2-hydroxy-N-[(1S)-1-hydroxy-3-oxopropyl]-L-aspartic acid | C7 H11 N O7 | 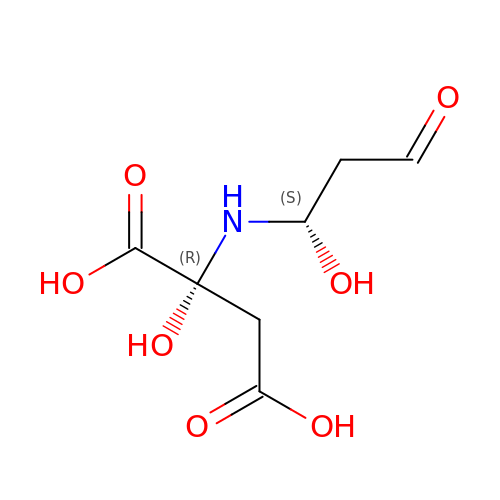CVFQCYNIQPQUNC-MHTLYPKNSA-N> MNKKQNFYAAIIVAIFLCLQLSHGSSGVSFEKTPAIKIVGNKFFDSESGEQFFIKGIAYQLQRSEEELSNANGAFETSYIDALA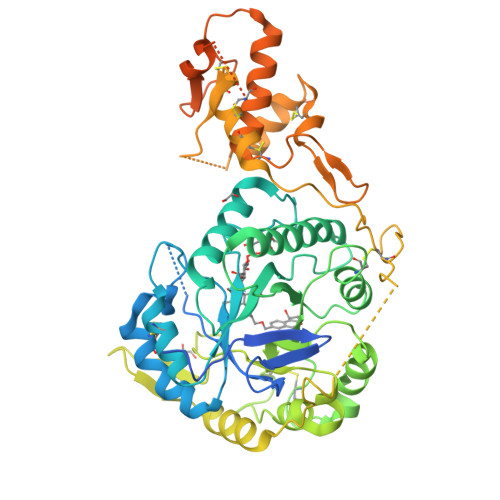DPKICLRDIPFLKMLGVNTLRVYAIDPTKSHDICMEALSAEGMYVLLDLSEPDISINRENPSWDVHIFERYKSVIDAMSSFPNLLGYFAGNEVTNDHTNTFASPFVKAAIRDAKEYISHSNHRKIPVGYSTNDDAMTRDNLARYFVCGDVKADFYGINMYEWCGYSTYGTSGYRERTKEFEGYPIPVFFSEFGCNLVRPRPFTEVSALYGNKMSSVWSGGLAYMYFEEENEYGVVKINDNDGVDILPDFKNLKKEFAKADPKGITEEEYLTAKEPTEVESVECPHIAVGVWEANEKLPETPDRSKCACLDEILPCEIVPFGAESGKYEEYFSYLCSKVDCSDILANGKTGEYGEFSDCSVEQKLSLQLSKLYCKIGANDRHCPLNDKNVYFNLESLQPLTSESICKNVFDSIRNITYNHGDYSKSNPSRSKESLNVKYPSSEERENDGTIAFKTSGFVILLISMIAAGILL(6R)-6-(pyridin-2-yl)-5,6-dihydrobenzimidazo[1,2-c]quinazoline 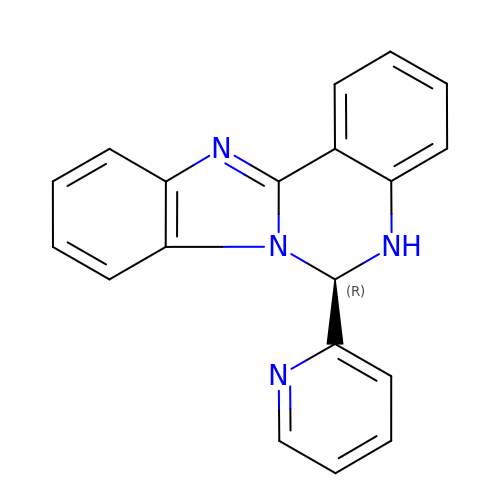| C19 H14 N4 | ZMZZAQWHHFSQPH-LJQANCHMSA-N>[3x]GAMVVKDQVDLRKRKHLEENERRHEDAIKRRKEAVNMNVEKPTVYHCKVFQFKNLQNPKIRFKLKMNSKELSLKGLCLRIRDDGPGIIIVVGNEKSCKFYENLVMKRIKWNEDFELHTNTGDIKMDMHNNSISKTWEGYLQDCKFKGWFMKVCNDQDSLLRTLGQFDSEHFYSPVQT

Except for an N-terminal region, Prp3 is highly conserved from yeast to human and contains a C-terminal domain of unknown function (DUF1115; PFAM ID PF06544). Here, we showed that Prp3 orthologs contain a C-terminal U4/U6 di-snRNA binding region that encompasses a DUF1115 domain and a preceding peptide rich in basic residues. Our crystal structure and targeted mutational analyses demonstrate that the DUF1115 domain acts as a ssRNA-binding domain that specifically recognizes the first 10 nts of the U6 3′-overhang. Our results indicate how Prp3 functionally bridges U4/U6 and U5 in the tri-snRNP by Prp3-RNA interactions on one side and Prp3-protein interactions on the other.

We therefore determined the crystal structure of yPrp3CTF at 2.7 Å resolution. The protein crystallized with three monomers per asymmetric unit. The electron density allowed modeling of residues 335–467, corresponding to the predicted DUF1115 domain. The structure exhibits a five-stranded mixed β-sheet with two α-helices (α1 and α2) running parallel to the β-strands on one side of the sheet and one (α3) on the other. The first 98 residues of the structure (residues 335–432) form a α/β sandwich with a ferredoxin-like topology and an additional, long β-hairpin (residues 403–421, comprising strands β3a and β3b) inserted between helix α2 and strand β4. The ferredoxin-like fold is further expanded by an extra β-strand (β5), a helix (α3) and a following loop at the C-terminus. In two of the three independent molecules, the β3a/β3b hairpins adopt very similar conformations with their long axes oriented perpendicular to the direction of the strands in the central β-sheet. Residues D405 and D418 at the bases of the hairpins coordinate an Yt3+ ion. To test whether the C-terminal U4/U6 di-snRNA-binding region is conserved in yPrp3, we produced a protein comprising the 177 C-terminal residues of yPrp3 (residue 296–469; yPrp3CTF). yPrp3CTF bound a yU4/U6 duplex containing the complete stem II and a 13-nt yU6 3′-overhang (yU4/U6stem II+13nt) with an apparent dissociation constant (Kd,app) of 0.92 µM as determined by EMSA (first gel and quantification) and with a Kd of 110 nM as determined by isothermal titration calorimetry (ITC).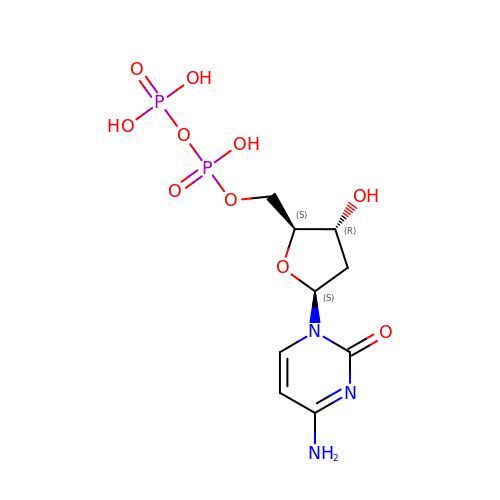4-amino-1-{2-deoxy-5-O-[(R)-hydroxy(phosphonooxy)phosphoryl]-beta-L-erythro-pentofuranosyl}pyrimidin-2(1H)-one | C9 H15 N3 O10 P2 | FTDHDKPUHBLBTL-CHKWXVPMSA-N1-tert-butyl-3-[(1H-indol-3-yl)methyl]-1H-pyrazolo[3,4-d]pyrimidin-4-amine | C18 H20 N6 | 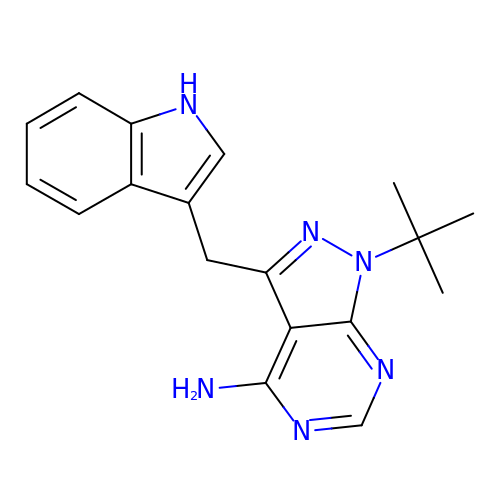WCMDCDJLTSDNJF-UHFFFAOYSA-N>[4x]HHHHHHGSMDKNIIIGAMTALITPFKNGKVDEQSYARLIKRQIENGIDAVVPVGTTGESATLTHEEHRTCIEIAVETCKGTKVKVLAGAGSNATHEAVGLAKFAKEHGADGILSVAPFYNKPTQQGLYEHYKAIAQSVDIPVLLYNVPGRTGCEISTDTIIKLFRDCENIYGVKEASGNIDKCVDLLAHE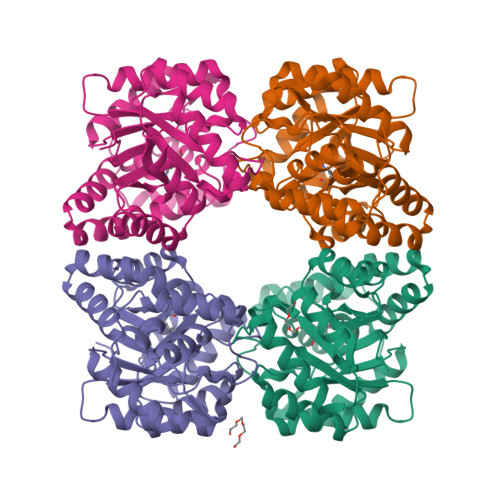PRMMLISGEDAINYPILSNGGKGVISVTSNLLPDMISALTHFALDENYKEAKKINDELYNINKILFCESNPIPIKTAMYLAGLIESLEFRLPLCSPSKENFAKIEEVMKKYKIKGF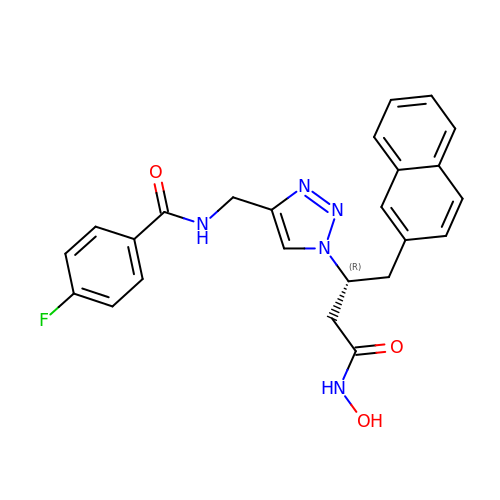4-fluoro-N-({1-[(2R)-4-(hydroxyamino)-1-(naphthalen-2-yl)-4-oxobutan-2-yl]-1H-1,2,3-triazol-4-yl}methyl)benzamide | C24 H22 F N5 O3 | RASCFMYPAZDCKQ-JOCHJYFZSA-N>[12x]MNIILKISGKF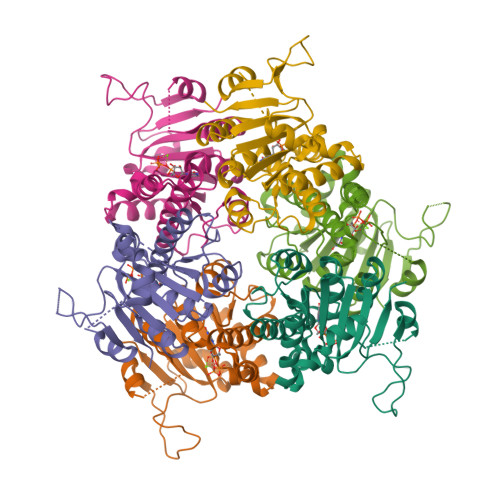FDEDNVDNLIVLRQSIKELADNGFRVGIVTGGGSTARRYIKLAREIGIGEAYLDLLGIWASRLNAYLVMFSLQDLAYMHVPQSLEEFIQDWSHGKVVVTGGFQPGQSTAAVAALVAEASSSKTLVVATNVDGVYEKDPRIYADVKLIPHLTTQDLRKILEGSQSVQAGTYELLDPLAIKIVERSKIRVIVMNYRKLNRIIDILKGEEVSSIIEPV> MSLLVDVLELLRPLLPSADTELTPDTELFSSQLLDSLALEEIQAAIESRWVP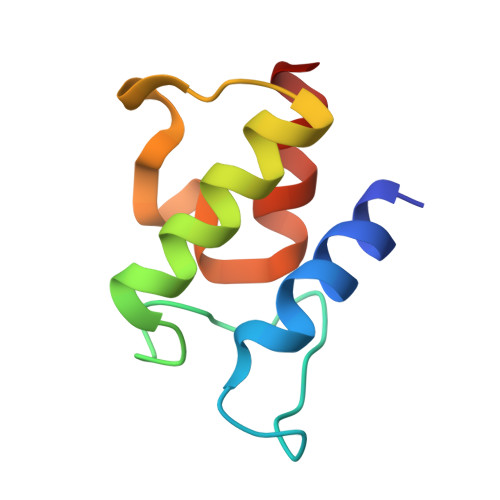LPPEELTLANFNTPAAIAETIARTST MENADIONE | C11 H8 O2 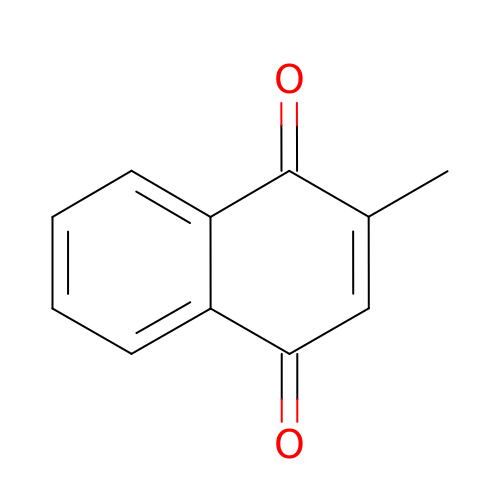| MJVAVZPDRWSRRC-UHFFFAOYSA-N>MRLWKAVVVTLAFVSTDVGVTTAIYAFSHLDRSLLEDIRHFNIFDSVLDLWAACLYRSCLLLGATIGVAKNSALGPRRLRASWLVITLVCLFVGIYAMAKLLLFSEVRRPIRDPWFWALFVWTYISLAASFLLWGLLATVRPDAEALEPGNEGFHGEGGAPAEQASGATLQKLLSYTKPDVAFLVAASFFLIVAALGETFLPYYTGRAIDSIVIQKSMDQFTTAVVVVCLLAIGSSLAAGIRGGIFTLVFARLNIRLRNCLFRSLVSQETSFFDENRTGDLISRLTSDTTMVSDLVSQNINIFLRNTVKVTGVVVFMFSLSWQLSLVTFMGFPIIMMVSNIYGKYYKRLSKEVQSALARASTTAEETISAMKTVRSFANEEEEAEVFLRKLQQVYKLNRKEAAAYMSYVWGSGLTLLVVQVSILYYGGHLVISGQMSSGNLIAFIIYEFVLGDCMESVGSVYSGLMQGVGAAEKVFEFIDRQPTMVHDGSLAPDHLEGRVDFENVTFTYRTRPHTQVLQNVSFSLSPGKVTALVGPSGSGKSSCVNILENFYPLQGGRVLLDGKPIGAYDHKYLHRVISLVSQEPVLFARSITDNISYGLPTVPFEMVVEAAQKANAHGFIMELQDGYSTETGEKGAQLSGGQKQRVAMARALVRNPPVLILDEATSALDAESEYLIQQAIHGNLQRHTVLIIAHRLSTVERAHLIVVLDKGRVVQQGTHQQLLAQGGLYAKLVQRQMLGLEHPLDYTASHKEPPSNTEHKA[2x]

TAPL is a lysosomal ATP-binding cassette transporter that translocates a broad spectrum of polypeptides from the cytoplasm into the lysosomal lumen. TAPL is a homodimeric half-transporter composed of a transmembrane domain (TMD) and a cytoplasmic nucleotide-binding domain (NBD) with an N-terminal TMD (TMD0). Here we report that, in addition to its well-known role as a peptide translocator, TAPL exhibits an ATP-dependent phosphatidylserine floppase activity that is the possible cause of its high basal ATPase activity and of the lack of coupling between ATP hydrolysis and peptide efflux. Here, we present the cryo-EM structures of mouse TAPL lacking the N-terminal TMD0 in (i) phospholipid-bound, (ii) both CHS- and 9-mer peptide-bound, and (iii) ADP·BeF3-bound states at 3.2–4.0 Å resolutions.

ΔTMD0 in nanodiscs was subjected to single-particle cryo-EM analysis in the absence of peptides and nucleotides. We obtained a 3D reconstruction with no preferred orientation of the particles at an overall 3.4 Å resolution. Monomers of ΔTMD0 assemble to form homodimers in which each monomer contains a TMD with six membrane-spanning α-helices (TM 5–10) and a cytoplasmic NBD. The protein adopts the canonical inward-facing conformation in which the transport pathway opens to the cytosol and the two NBDs remain separate. However, ΔTMD0 has a cylinder-shaped transport pathway in which the highly conserved F449 residues on TM 10 penetrate into the transport pathway and face each other, forming the narrowest point (7.5 Å). Consequently, ΔTMD0 has two separate substrate binding sites, a central cavity in the cytosolic leaflet of the lysosomal membrane and an upper cavity in the luminal leaflet. The shape of the density clearly corresponds to a phospholipid molecule with two fatty acyl chains. Also, cardiolipins with four acyl chains cannot fit on the map. We, therefore, built an atomic model of the PG (16:0–18:0) molecule in the head-up direction as a phospholipid model. The bound PG mainly interacts through hydrophobic interactions between the lipid acyl chains and non-polar residues of both monomers, including L201, V227, L424, I442, I445, I446, F449, and V450. The inward-facing ΔTMD0 structure has a wide lateral gate facing the cytosolic leaflet of the lysosomal membrane, with an opening of ~18 Å in the largest diameter.>[2x]SNSADETLCQT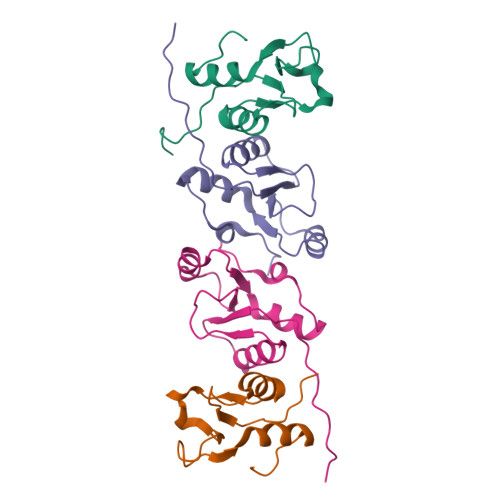KVLLDIFTGVRLYLPPSTPDFSRLRRYFVAFDGDLVQEFDMTSATHVLGSRDKNPAAQQVSPEWIWACIRKRRLVAPS;>MQEPPDLPVPELPDFFEGKHFFLYGEFPGDERRRLIRYVTAFNGELEDRMNERVQFVITAQEWDPNFEEALMENPSLAFVRPRWIYSCNEKQKLLPHQLYGVVPQA[2x]>[4x]MSLEAIVFDRSEPENVSVKVLDQLLLPYTTKYVPIHTIDDGYSVIKSMQVRGAPAIAIVGSLSVLTEVQLIKHNPTSDVATLYSLVNWESTKTVLNKRLDFLLSSRPTAVNLSNSLVEIKNILKSSSDLKAFDGSLYNYVCELIDEDLANNMKMGDNGAKYLIDVLQKDGFKDEFAVLTICNTGSLATSGYGTALGVIRSLWKDSLAKTDK;>CPRMGHVFPLETRPYNQGSRLTAYELVYDKI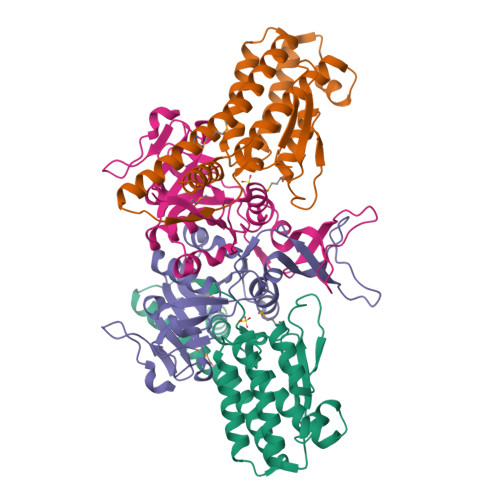PSTLITDSSIAYRIRTSPIPIKAAFVGADRIVRNGDTANKIGTLQLAVICKQFGIKFFVVAPKTTIDNVTETGDDIIVEERNPEEFKVVTGTVINPENGSLILNESGEPITGKVGIAPLEINVWNPAFDITPHELIDGIITEEGVFTKNSSGEFQLESLF[4x]undecyl 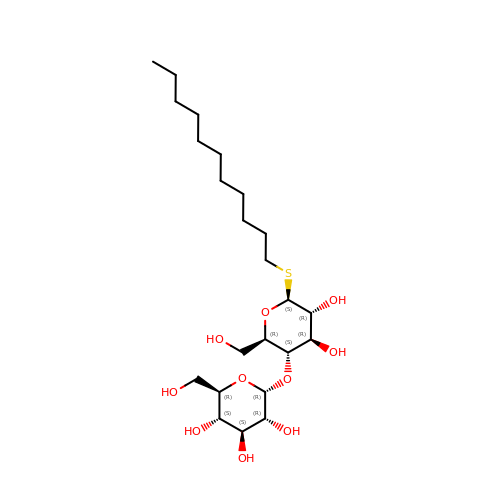4-O-alpha-D-glucopyranosyl-1-thio-beta-D-glucopyranoside | C23 H44 O10 S | SQISXDUZDUDUNY-GNKAUAAYSA-N> MGSSH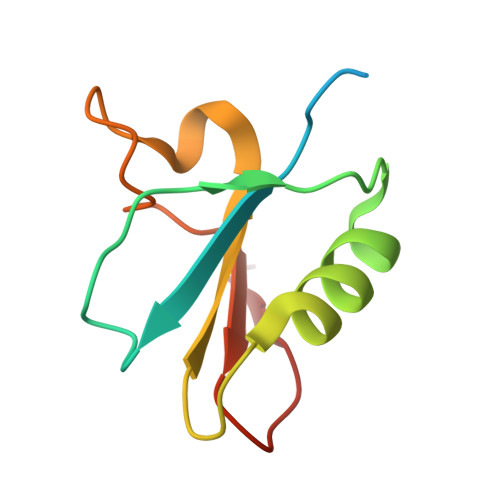HHHHHSQDPMTNVVYYFTETNNINAYATAEALKAQTLADAKREASRRQCFQGTTLKIGTIYSLNSDGLLVDEITSKEDGKKWVDRY>[4x]MWKDKEFQVLFVLTILTLISGTIFYSTVEGLRPIDALY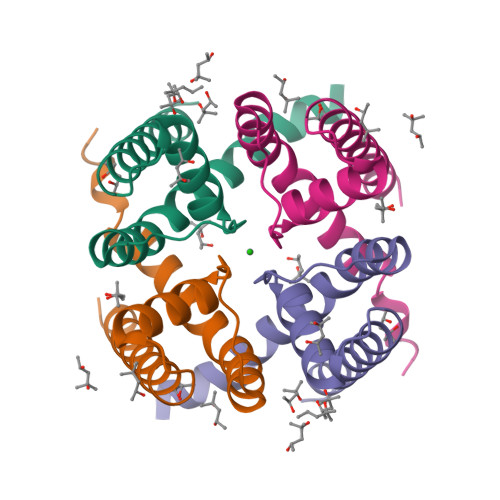FSVVTLTTVGCDISPQTDFGKIFTILYIFIGIGLVFGFIHKLAVNVQLPSILSNLVPR>[3x]MEPHVLGAVLYWLLLPCALLAACLLRFSGLSLVYLLFLLLLPWFPGPTRCGLQGHTGRLLRALLGLSLLFLVAHLALQICLHIVPRLDQLLGPSCSRWETLSRHIGVTRLDLKDIPNAIRLVAPDLGILVVSSVCLGICGRLARNTRQSPHPRELDDDERDVDASPTAGLQEAATLAPTRRSRLAARFRVTAHWLLVAAGRVLAVTLLALAGIAHPSALSSVYLLLFLALCTWWACHFPISTRGFSRLCVAVGCFGAGHLICLYCYQMPLAQALLPPAGIWARVLGLKDFVGPTNCSSPHALVLNTGLDWPVYASPGVLLLLCYATASLRKLRAYRPSGQRKEAAKGYEARELELAELDQWPQERESDQHVVPTAPDTEADNCIVHELTGQSSVLRRPVRPKRAEPREASPLHSLGHLIMDQSYVCALIAMMVWSITYHSWLTFVLLLWACLIWTVRSRHQLAMLCSPCILLYGMTLCCLRYVWAMDLRPELPTTLGPVSLRQLGLEHTRYPCLDLGAMLLYTLTFWLLLRQFVKEKLLKWAESPAALTEVTVADTEPTRTQTLLQSLGELVKGVYAKYWIYVCAGMFIVVSFAGRLVVYKIVYMFLFLLCLTLFQVYYSLWRKLLKAFWWLVVAYTMLVLIAVYTFQFQDFPAYWRNLTGFTDEQLGDLGLEQFSVSELFSSILVPGFFLLACILQLHYFHRPFMQLTDMEHVSLPGTRLPRWAHRQDAVSGTPLLREEQQEHQQQQQEEEEEEEDSRDEGLGVATPHQATQVPEGAAKWGLVAERLLELAAGFSDVLSRVQVFLRRLLELHVFKLVALYTVWVALKEVSVMNLLLVVLWAFALPYPRFRPMASCLSTVWTCVIIVCKMLYQLKVVNPQEYSSNCTEPFPNSTNLLPTEISQSLLYRGPVDPANWFGVRKGFPNLGYIQNHLQVLLLLVFEAIVYRRQEHYRRQHQLAPLPAQAVFASGTRQQLDQDLLGCLKYFINFFFYKFGLEICFLMAVNVIGQRMNFLVTLHGCWLVAILTRRHRQAIARLWPNYCLFLALFLLYQYLLCLGMPPALCIDYPWRWSRAVPMNSALIKWLYLPDFFRAPNSTNLISDFLLLLCASQQWQVFSAERTEEWQRMAGVNTDRLEPLRGEPNPVPNFIHCRSYLDMLKVAVFRYLFWLVLVVVFVTGA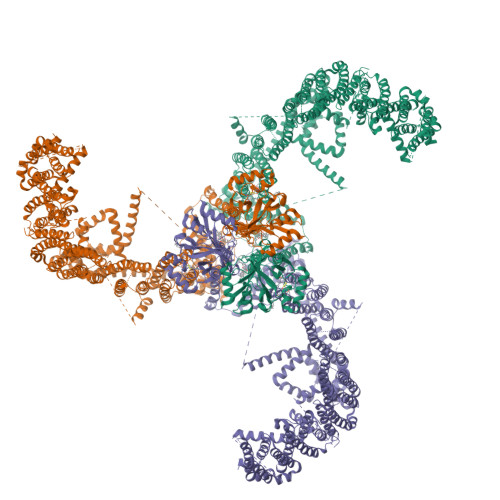TRISIFGLGYLLACFYLLLFGTALLQRDTRARLVLWDCLILYNVTVIISKNMLSLLACVFVEQMQTGFCWVIQLFSLVCTVKGYYDPKEMMDRDQDCLLPVEEAGIIWDSVCFFFLLLQRRVFLSHYYLHVRADLQATALLASRGFALYNAANLKSIDFHRRIEEKSLAQLKRQMERIRAKQEKHRQGRVDRSRPQDTLGPKDPGLEPGPDSPGGSSPPRRQWWRPWLDHATVIHSGDYFLFESDSEEEEEAVPEDPRPSAQSAFQLAYQAWVTNAQAVLRRRQQEQEQARQEQAGQLPTGGGPSQEVEPAEGPEEAAAGRSHVVQRVLSTAQFLWMLGQALVDELTRWLQEFTRHHGTMSDVLRAERYLLTQELLQGGEVHRGVLDQLYTSQAEATLPGPTEAPNAPSTVSSGLGAEEPLSSMTDDMGSPLSTGYHTRSGSEEAVTDPGEREAGASLYQGLMRTASELLLDRRLRIPELEEAELFAEGQGRALRLLRAVYQCVAAHSELLCYFIIILNHMVTASAGSLVLPVLVFLWAMLSIPRPSKRFWMTAIVFTEIAVVVKYLFQFGFFPWNSHVVLRRYENKPYFPPRILGLEKTDGYIKYDLVQLMALFFHRSQLLCYGLWDHEEDSPSKEHDKSGEEEQGAEEGPGVPAATTEDHIQVEARVGPTDGTPEPQVELRPRDTRRISLRFRRRKKEGPARKGAAAIEAEDREEEEGEEEKEAPTGREKRPSRSGGRVRAAGRRLQGFCLSLAQGTYRPLRRFFHDILHTKYRAATDVYALMFLADVVDFIIIIFGFWAFGKHSAATDITSSLSDDQVPEAFLVMLLIQFSTMVVDRALYLRKTVLGKLAFQVALVLAIHLWMFFILPAVTERMFNQNVVAQLWYFVKCIYFALSAYQIRCGYPTRILGNFLTKKYNHLNLFLFQGFRLVPFLVELRAVMDWVWTDTTLSLSSWMCVEDIYANIFIIKCSRETEKKYPQPKGQKKKKIVKYGMGGLIILFLIAIIWFPLLFMSLVRSVVGVVNQPIDVTVTLKLGGYEPLFTMSAQQPSIIPFTAQAYEELSRQFDPQPLAMQFISQYSPEDIVTAQIEGSSGALWRISPPSRAQMKRELYNGTADITLRFTWNFQRDLAKGGTVEYANEKHMLALAPNSTARRQLASLLEGTSDQSVVIPNLFPKYIRAPNGPEANPVKQLQPNEEADYLGVRIQLRREQGAGATGFLEWWVIELQECRTDCNLLPMVIFSDKVSPPSLGFLAGYGIMGLYVSIVLVIGKFVRGFFSEISHSIMFEELPCVDRILKLCQDIFLVRETRELELEEELYAKLIFLYRSPETMIKWTREKE> AWPKVQPEVNIGVVGHV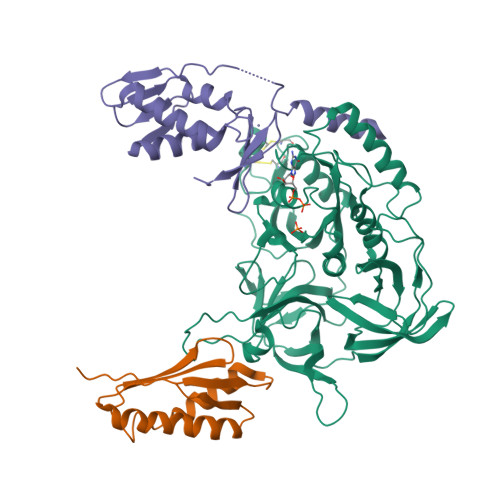DHGKTTLVQAITGIWTSKHSEELKRGMTIKLGYAETNIGVCESCKKPEAYVTEPSCKSCGSDDEPKFLRRISFIDAPGHEVLMATMLSGAALMDGAILVVAANEPFPQPQTREHFVALGIIGVKNLIIVQNKVDVVSKEEALSQYRQIKQFTKGTWAENVPIIPVSALHKINIDSLIEGIEEYIKTPYRDLSQKPVMLVIRSFDVNKPGTQFNELKGGVIGGSIIQGLFKVDQEIKVLPGLRVEKQGKVSYEPIFTKISSIRFGDEEFKEAKPGGLVAIGTYLDPSLTKADNLLGSIITLADAEVPVLWNIRIKYNLLERVVGAKEMLKVDPIRAKETLMLSVGSSTTLGIVTSVKKDEIEVELRRPVAVWSNNIRTVISRQIAGRWRMIGWGLVEI;> MRKVKMSGLITVRTNEPLGVEKIKEVISKALENIEQDYESLLNIKIYTIGAPRYRVDVVGTNPKEASEALNQIISNLIKIGKEENVDISVVKK;> SSEKEYVEMLDRLYSKLPEKGRKEGTQSLPNMIILNIGNTTIIRNFAEYCDRIRREDKICMKYLLKELAAPGNVDDKGELVIQGKFSSQVINTLMERFLKAYVECSTCKSLDTILKKEKKSWYIVCLACGAQTPVKPL>[6x]NNELSPVALRQMSCAAGTTQTA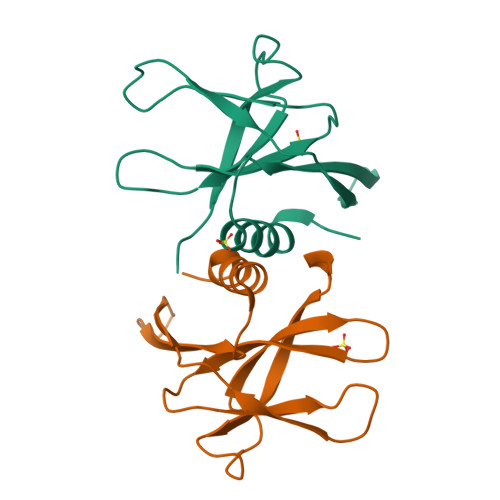CTDDNALAYYNTTKGGRFVLALLSDLQDLKWARFPKSDGTGTIYTELEPPCRFVTDTPKGPKVKYLYFIKGLNNLNRGMVLGSLAATVRLQ> MDLEKNYPTPRTSRTGHGGVNQLGGVFVNGRPLPDVVRQRIVELAHQGVRPCDISRQLRVSHGCVSKILGRYYETGSIKPGVIGGSKPKVATPKVVEKIAEYKRQNPTMFAWEIRDRLLAERVCDNDTVPSVSSINRIIRTKVQQPPNQ;> VPSYDSFDYEDYPAALPNHKPKGTFKDY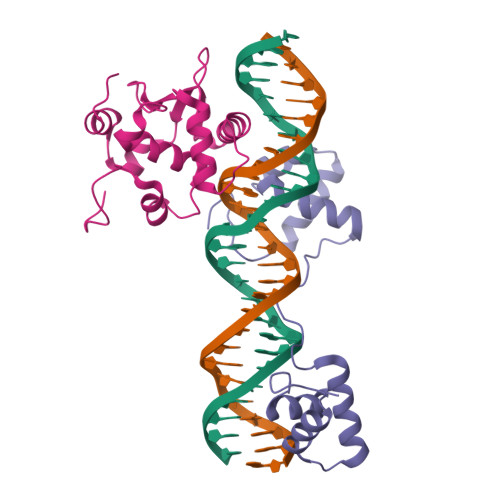VRDRADLNKDKPVIPAAALAGYTGSGPIQLWQFLLELLTDKSCQSFISWTGDGWEFKLSDPDEVARRWGKRKNKPKMNYEKLSRGLRYYYDKNIIHKTAGKRYVYRFVCDLQSLLGYTPEELHAMLDVKPDAD(3E)-N~8~-(2-aminophenyl)-N~1~-phenyloct-3-enediamide | C20 H23 N3 O2 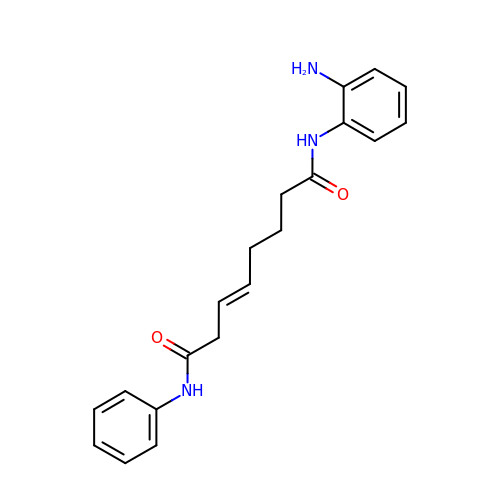| WWKBRKDVEBSJBW-LZCJLJQNSA-N> LAAAEEYIATFKGSEYFCYDLSQNPIQSSSDEITLSFKTLQRNGLMLHTGKSADYVNLALKNGAVSLVINLGSGAFEALVEPVNGKFNDNAWHDVKVTRNLRQVTISVDGILTTTGYTQEDYTMLGSDDFFYVGGSPSTADLPGSPVSNNFMGCLKEVVYKNNDVRLELSRLAKQGDPKMKIHGVVAFKCENVATLDPITFETPESFISLPKWNAKKTGSISFDFRTTEPNGLILFSHGKPRHQKDAKHPQMIKVDFFAIEMLDGHLYLLLDMGSGTIKIKALQKKVNDGEWYHVDFQRDGRSGTISVNTLRTPYTAPGESEILDLDDELYLGGLPENKAGLVFPTEVWTALLNYGYVGCIRDLFIDGQSKDIRQMAEVQSTAGVKPSCSRETAKPCLSNPCKNNGMCRDGWNRYVCDCSGTGYLGRSCEREATVLSYDGSMFMKIQLPVVMHTEAEDVSLRFRSQRAYGILMATTSRDSADTLRLELDAGRVKLTVNLDCIRINCNSSKGPETLFAGYNLNDNEWHTVRVVRRGKSLKLTVDDQQAMTGQMAGDHTRLEFHNIETGIITERRYLSSVPSNFIGHLQSLTFNGMAYIDLCKNGDIDYCELNARFGFRNIIADPVTFKTKSSYVALATLQAYTSMHLFFQFKTTSLDGLILYNSGDGNDFIVVELVKGYLHYVFDLGNGANLIKGSSNKPLNDNQWHNVMISRDTSNLHTVKIDTKITTQITAGARNLDLKSDLYIGGVAKETYKSLPKLVHAKEGFQGCLASVDLNGRLPDLISDALFCNGQIERGCEGPSTTCQEDSCSNQGVCLQQWDGFSCDCSMTSFSGPLCNDPGTTYIFSKGGGQITYKWPPNDRPS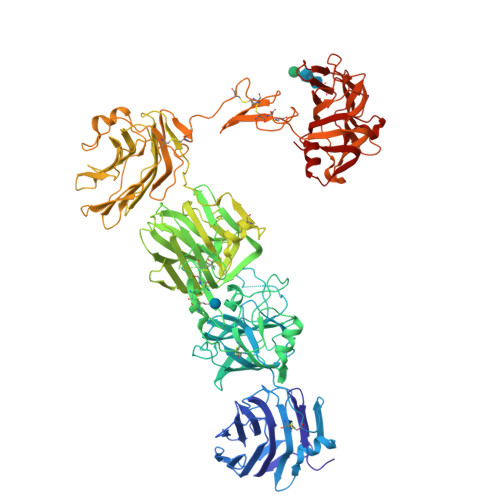TRADRLAIGFSTVQKEAVLVRVDSSSGLGDYLELHIHQGKIGVKFNVGTDDIAIEESNAIINDGKYHVVRFTRSGGNATLQVDSWPVIERYPAGRQLTIFNSQATIIIGGKEQGQPFQGQLSGLYYNGLKVLNMAAENDANIAIVGNVRLLEVLFQ>MIPVTELRYFADTQPAYRILKPWWDVFTDYISIVMLMIAVFGGTLQVTQDKMICLPCKWVTKDSCNDSFRGWAAPGPEPTYPNSTILPTPDTGPTGIKYDLDRHQYNYVDAVCYENRLHWFAKYFPYLVLLHTLIFLACSNFWFKFPRTSSKLEHFVSILLKCFDSPWTTRALSETVVEESDPKPAFSKMNGSMDKKSSTVSEDVEATVPMLQRTKSRIEQGIVDRSETGVLDKKEGEQAKALFEKVKKFRTHVEEGDIVYRLYMRQTIIKVIKFILIICYTVYYVHNIKFDVDCTVDIESLTGYRTYRCAHPLATLFKILASFYISLVIFYGLICMYTLWWMLRRSLKKYSFESIREESSYSDIPDVKNDFAFMLHLIDQYDPLYSKRFAVFLSEVSENKLRQLNLNNEWTLDKLRQRLTKNAQDKLELHLFMLSGIPDTVFDLVELEVLKLELIPDVTIPPSIAQLTGLKELWLYHTAAKIEAPALAFLRENLRALHIKFTDIKEIPLWIYSLKTLEELHLTGNLSAENNRYIVIDGLRELKRLKVLRLKSNLSKLPQVVTDVGVHLQKLSINNEGTKLIVLNSLKKMANL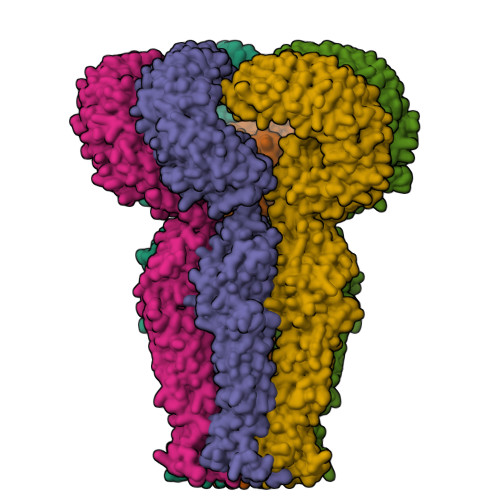TELELIRCDLERIPHSIFSLHNLQEIDLKDNNLKTIEEIISFQHLHRLTCLKLWYNHIAYIPIQIGNLTNLERLYLNRNKIEKIPTQLFYCRKLRYLDLSHNNLTFLPADIGLLQNLQNLAITANRIETLPPELFQCRKLRALHLGNNVLQSLPSRVGELTNLTQIELRGNRLECLPVELGECPLLKRSGLVVEEDLFNTLPPEVKERLWRADKEQA[6x]Malonyl-CoA reductase (MCR) is a NADPH-dependent bi-functional enzyme that performs alcohol dehydrogenase and aldehyde dehydrogenase (CoA-acylating) activities in the N- and C-terminal fragments, respectively. It catalyzes the two-step reduction of malonyl-CoA to 3-hydroxypropionate (3-HP), a key reaction in the autotrophic CO2 fixation cycles of Chloroflexaceae green non-sulfur bacteria and the archaea Crenarchaeota. In contrast, green non-sulfur bacteria, including members of the genera Chloroflexus and Roseiflexus, employ a single bi-functional MCR to catalyze both reduction reactions of malonyl-CoA. Full-length RfxMCR was a homodimer of two cross-interlocked subunits, each containing four tandemly arranged short-chain dehydrogenase/reductase (SDR) domains.

The crystal structure of RfxMCR-C in complex with NADP+–MSA was also determined by the molecular replacement method and reﬁned to an Rwork of 22.05% and an Rfree of 25.28% at 2.3 Å resolution. The overall structure contained 28 α-helixes and 13 β-strands that were organized into tandemly arranged SDR3 (Gly573–Glu782 and Met933–Gly962), ED (Leu783–Thr932), and SDR4 (Phe963–Val1229) domains. Similar to RfxMCR-N, a cofactor NADP+ and intermediate MSA were resolved at the interface between the SDR3 and ED domains. In the substrate-binding pocket, MSA was immobilized by hydrogen bonding interactions with Ser731 (3.0 Å) and Tyr749 (3.2 Å) from the SDR3 domain and Arg799 (3.5 Å) from the ED. NADP+ was coordinated in the cofactor-binding pocket through extensive hydrogen bonding interactions with Tyr749 (2.6 Å), Lys753 (3.1 Å), Ser593 (2.7 Å), Arg616 (2.9 Å), and Asp651 (3.2 Å). Mutation of the NADP+–MSA coordinating residues Ser731, Tyr749, Lys753, and Arg799 completely eliminated enzymatic activity. When NADP+–MSA was bound, members of the SDR3 catalytic triad (Ser731–Lys753–Tyr749) were shifted toward the substrate-binding pocket to form hydrogen bonds with NADP+ and MSA. Specifically, the guanidine side chain of Arg799 was flipped by ~1.6 Å to stabilize the MSA carbonyl group, and the side chains of Asp651 and Arg616 were shifted by ~2.0 Å and 4.1 Å, respectively, to immobilize the adenosine ring of NADP+; this further resulted in partial closure of the adenosine ring–binding site in NADP+–MSA-bound RfxMCR-C. As indicated in the structural analyses of NADP+–MSA-bound RfxMCR-C, the reaction intermediate MSA could be further stabilized in a proton relay network by hydrogen bonding interactions with Ser731, Tyr749, and Arg799 for the second reduction step.

> MGSSHHHHHHGWAESLFGLHMGKVALITGGSAGIGGQIGRLLALSGAHVMLAARNADQLEQMRASIVREVRDASYPDAESRVAIFPGSDVSDIDGLERLVNHTVRVFGKVDYLINNAGIAGAEEMVIDMPVDAWRHTLRANLISNYALLRRLAPQMKAAGGAYVLNVSSYFGGEKYVAIPYPNRSDYAVSKAGQRAMVESLARFLGPEIQINAIAPGPVEGERLKGAGSRPGLFMRRARLILENKRLNEVFAALLAARHEGATIADLLPDLFANDIQSIANSAAMPAPLRRLATMLRETSDAGGSAQSYLMNATIARKLLNRLENGGYITLHDRRALTVEPPEPFFTEAQIEREAIKVRDGILGMLHLQRMPTEFDVALATVFYLADRNVTGETFHPSGGLRFERTVTEGELFGKPGQQRLERLKGSVVYLIGEHLRQHLVLLARTFLDEIHVARVVLLTETTQAATDLAAELSDYEAAGRFVVIPTCGDIEGGIDRAMAEYGRPGPVISTPFRPLPDRALSARNGDWSSVLTTAEFEELVEQQITHHFRVARKAGLIEGANVTLVTPPTSARSTSEEFALANFVKTTLHALTATAGAESERTVPHVPVNQVDLTRRARSEEPRTPSEEEEELQRFVNAVLLTSAPLPTPLESRYRARIYRGNAITV[4-[3-(DIFLUORO-PHOSPHONO-METHYL)PHENYL]PHENYL]METHOXYAZANIUM | 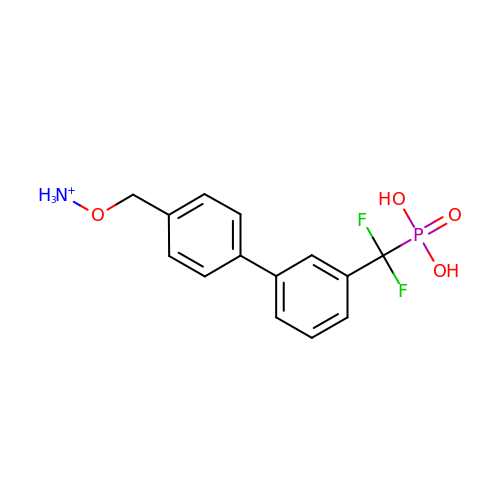C14 H15 F2 N O4 P | FWYIUZIHUWHORI-UHFFFAOYSA-O>[2x]DLGAPQNPNAK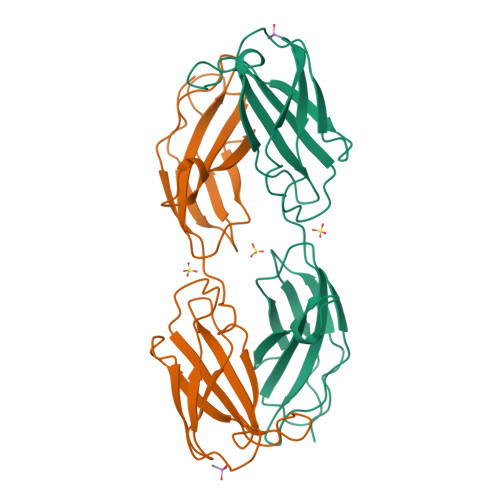AAGSRKIHFNWLPPSGKPMGYRVKYWIQGDSESEAHLLDSKVPSVELTNLYPYCDYEMKVCAYGAQGEGPYSSLVSCRTHQEVPSEPGRLAFNVVSSTVTQLSWAEPAETNGEITAYEVCYGLVNDDNRPIGPMKKVLVDNPKNRMLLIENLRESQPYRYTVKARNGAGWGPEREAIINLATQP>MSEAVERNYDPGDVAIIGASCRFPGARNKEQYWDNLLHGREGVTFYAKDEIEVDETLINSPAYVRATGALDGYDEFDPAVFGVSDRMAAAMTPEHRVFLEASWEVMEDASYDPERVRGEVGVYASTNPQSAALYSSPPDWVSAGPEVMDRSNAWLPDTITSNVLYYLGLTGEAVTVTAVCSGFHYAVHLACQSLLLGQTDMAIAGGVMVRLPQRRGYLWEEGRILSRDGHCRPFDANGTGSVLASGVAVVLLKPLPQAVADRDHIYATVKGTAINNNGISAMAYGLAQPERLSACIAGAMQAGDVAPETVSMYEANGFGMPITDSLEVHAAHLAFGKQSGTCSIGAVKGNIGHAGVVAGGSGAVKAAFALYHRSLPPTINLTELNEEIDFPRTPFVPQLEPAAWQPECGIRRAGITALGGGGYNAHLVLEEPPRPVEREPENRRPRIVTLSALDD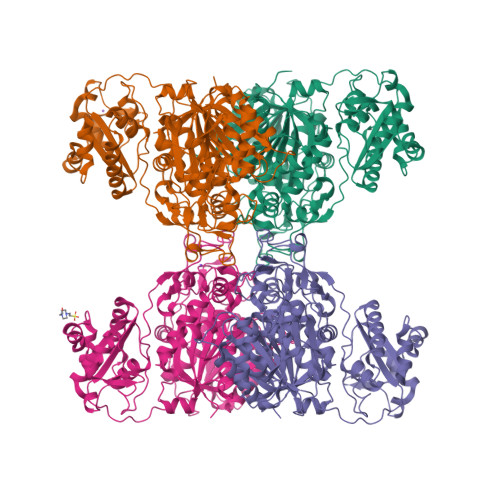AAVSRQRAALSSWLAEHSDARLDDIAYSLNLGRKALPSRWAAVISTRDELLEVLSGDGKSGRVSRFGQERRADLARFRRTEDGLALGSGDEMRDVQALTELAAAWVQGERVNFEVLHADERSHRISLPNYPFARRRFWRTDW[4x]(1R,3S,5Z)-5-[(2E)-2-{(1R,3aS,7aR)-1-[(1R,5S)-5-hydroxy-1-methyl-5-(1,3-thiazol-2-yl)pentyl]-7a-methyloctahydro-4H-inden-4-ylidene}ethylidene]-4-methylidenecyclohexane-1,3-diol 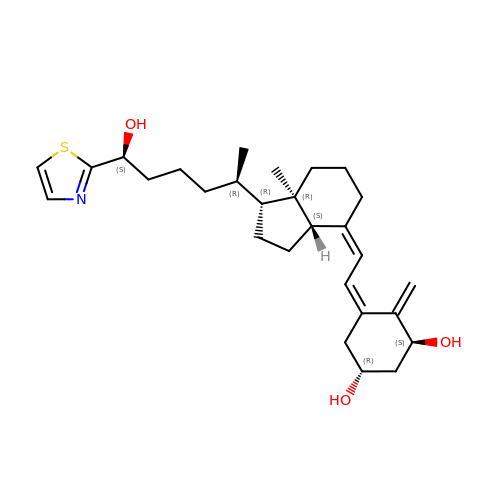| C28 H41 N O3 S | AZVJHDPZXYTKQV-LCRUICLWSA-N> MTTPSMEDYIEQIYMLIEEKGYARVSDIAEALAVHPSSVTKMVQKLDKDEYLIYEKYRGLVLTSKGKKIGKRLVYRHELLEQFLRI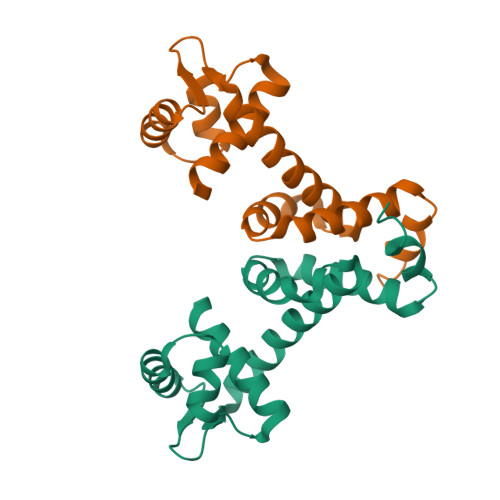IGVDEEKIYNDVEGIEHHLSWNSIDRIGDLVQYFEEDDARKKDLKSIQKKTEHHNQ> MTYIVGLTGGIGSGKTTIANLFTDLGVPLVDADVVAREVVAKDSPLLSKIVEHFGAQILTEQGELNRAALRERVFNHDEDKLWLNNLLHPAIRERMKQKLAEQTAPYTLFVVPLLIENKLTALCDRILVVDVSPQTQLARSAQRDNNNFEQIQRIMNSQVSQQERLKWADD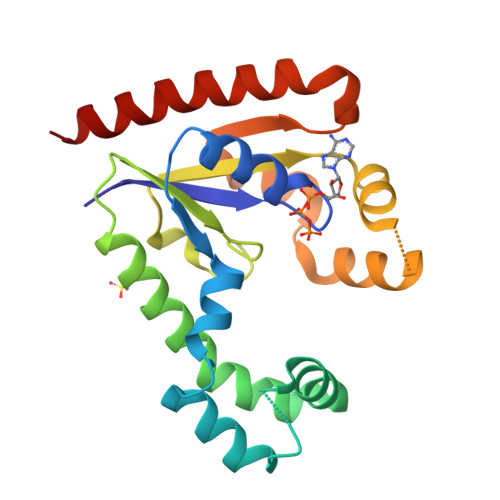VINNDAELAQNLPHLQQKVLELHQFYLQQAENKNA>[2x]MLVVGSELQSDAQQLSAEAPRHGELQYLRQVEHILRCGFKKEDRTGTGTLSVFGMQARYSLRDEFPLLTTKRVFWKGVLEELLWFIKGSTNAKELSSKGVRI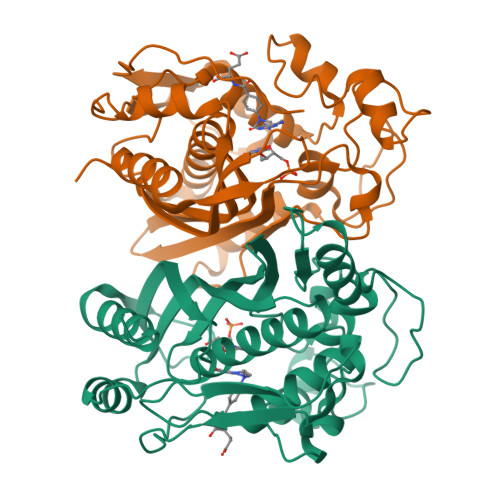WDANGSRDFLDSLGFSARQEGDLGPVYGFQWRHFGAEYKDMDSDYSGQGVDQLQKVIDTIKTNPDDRRIIMCAWNPKDLPLMALPPCHALCQFYVVNGELSCQLYQRSGDMGLGVPFNIASYALLTYMIAHITGLQPGDFVHTLGDAHIYLNHIEPLKIQLQREPRPFPKLKILRKVETIDDFKVEDFQIEGYNPHPTIKMEMAV>MGTEESKQRVIQEYVPGKQVTLAHIIANPNEDIYKKLGLVLDKKDAIGILTITPSEASIIAADVATKASNVSLGFIDRFSGSVVISGDVSSVESALNDVLEVLGNMLNFSSTKITRTLEHHHHHH[2x]

To understand the structure and function of the C. difficile eut bacterial microcompartment we have determined the crystal structures of two proteins with homology to BMC shell proteins, CD1908 and CD1918, and show that they are well conserved between species. We have also determined the atomic structure of CD1925, a member of the EutQ family of cupin barrels. The sequestration of ethanolamine metabolism within a BMC is thought to protect the cell from the acetaldehyde produced as an intermediate in its breakdown and to prevent the loss of this volatile compound and its carbon from the cell.

The structure of CD1908 was determined by molecular replacement to 1.51 Å resolution. Two molecules are present in the asymmetric unit, comprising the complete native protein sequence, less the N-terminal methionine, with a single amino acid visible from the C-terminal His6 tag in chain A. CD1908 displays a permuted BMC domain fold, with a four-stranded anti-parallel β-sheet flanked by two α-helices on one face and one helix on the other with an N-terminal β-strand extension. The protein forms a hexamer with pairs of molecules related by the crystallographic 3-fold axis. A glycerol molecule from the crystallisation condition was found associated with each chain. The N-terminal face of CD1908 has distinct patterns of positive charge on the surface, with a shallow depression at the centre of the oligomer that is approximately 10 Å in diameter and blocked by Glu11. The opposite face of the protein has a distinct conical cavity that is 25 Å wide at its widest point and has Glu11 at its apex (Fig. 5B/C). The role that CD1908 may play in the structure of the BMC shell is not clear; unlike EutS, which is able to form enclosed compartments when over-expressed alone in E. coli, CD1908 and its homologue PduU form no higher order structures.> ATIVALKYPGGVVMAGDRRSTQGNMISGRDVRKVYITDDYTATGIAGTAAVAVEFARLY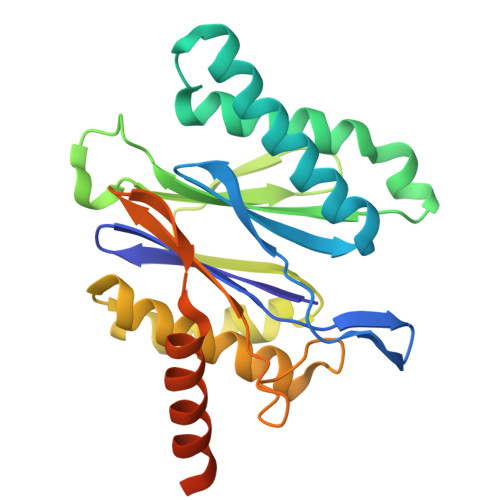AVELEHYEKLEGVPLTFAGKINRLAIMVRGNLAAAMQGLLALPLLAGYDIHASDPQSAGRIVSFDAAGGWNIEEEGYQAVGSGSLFAKSSMKKLYSQVTDGDSGLRVAVEALYDAADDDSATGGPDLVRGIFPTAVIIDADGAVDVPESRIAELARAIIESRSGADTFGSDGGEKWSHPQFEK> IATLVERSLEKHKDRLFDCGASGQPVTYKEVAEHARSISETLKAAAAYLHVPLTLPSALGRAGADGQARHTATSTEDCTGSASTLKCRGKPLNRPTIGLIVPPNSVAILAHLVGVWQCGGVGLLLPFPDPACLPFVADSTAAAAASAANAAVLFAKGGKTLHTYRPDALFQGNTGPSVYAKTVNPNSLPFLNSQNNAHNRNGVAQLWEYQAAESRCHLLVVTPEVAPMAAEVASKLSIPICVLRTSWVRKSDGTNGAEEQRAPERDLWSVRGRNKLEVKAYVPEVFHDSSRTSRNITRWQLLEVTPHECTHAAADEESIAEVAAPATHFFQGPAAHAPRAVIYSHKALSDQVIRNKDLLQL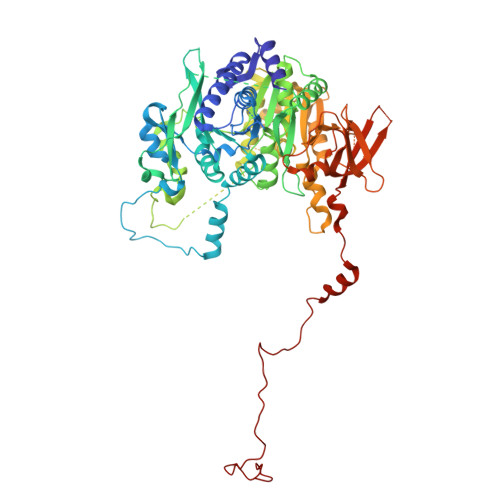NAEDHVVILHLPFFGSHRSGTGSQASSRMLCTPKGLVAVAMPAVAAGSTLSFLSSSDKIQDSLLPLPLQLQRLQDRLPQNEKIPRQPEQRQALLPLGCDIPEKTPWRCSGTTTRGPLVPRGNQEGLQVDFTGAYENTLEVNALQMWEKIASLHEDGRNTTRSRKQRFTSRDKATPELSRQATVLAMDAETAATMVQVIATERFQMEGTNEKAHASGGSDASRFPTITSKDITRYKAAVKSLRLICICTDEGDLGASFSGRWSSSNKGGGIRIQSLLRSLQALAGPDTKILHLCSLTETGLLMVGGPLPDGSPGSRERGEKSDFGEPLQDHLSTGCKDSKTQCLDATDGEDRANFTGVVAPGIKVEIDDETDQLRVRSGHMAMGFHGRPRSTQESFDSAGLFRSSFGGSLVTNRRNDTDIIGCDRGEAEQRVELFKCVYSAAVPRLPLLHRLIASFKNSPKMESHIEGYVKKKPIAGRDWNNLHAPRKHWKKMFL>[6x]MKP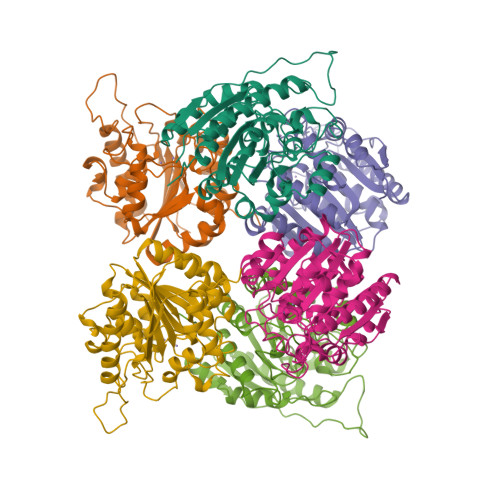ISIIGVPMDLGQTRRGVDMGPSAMRYAGVIERLERLHYDIEDLGDIPIGKAERLHEQGDSRLRNLKAVAEANEKLAAAVDQVVQRGRFPLVLGGDHSIAIGTLAGVAKHYERLGVIWYDAHGDVNTAETSPSGNIHGMPLAASLGFGHPALTQIGGYSPKIKPEHVVLIGVRSLDEGEKKFIREKGIKIYTMHEVDRLGMTRVMEETIAYLKERTDGVHLSLDLDGLDPSDAPGVGTPVIGGLTYRESHLAMEMLAEAQIITSAEFVEVNPILDERNKTASVAVALMGSLFGEKLM> LITDPRSGRTYLKGRLLGKGGFARCYEATDTETGSAYAVKVIPQSRVAKPHQREKILNEIELHRDLQHRHIVRFSHHFEDADNIYIFLELCSRKSLAHIWKARHTLLEPEVRYYLRQILSGLKYLHQRGILHRDLKLGNFFITENMELKVGDFGLAARLEPPEQRKKTICGTPNYVAPEVLLRQGHGPEADVWSLGCVMYTLLCGSPPFETADLKETYRCIKQVHYTLPASLSLPARQLL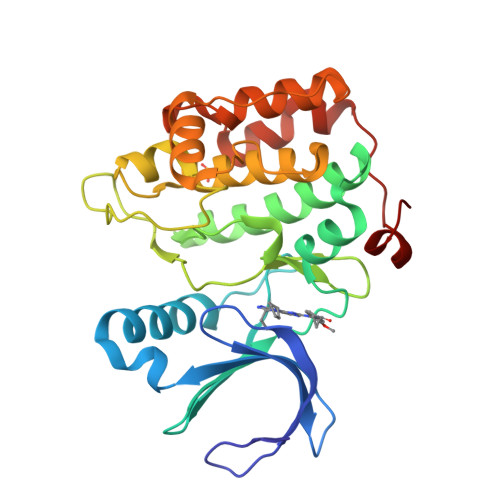AAILRASPRDRPSIDQILRHDFFTKGYTPDRLPISSCVTVP>[3x]PF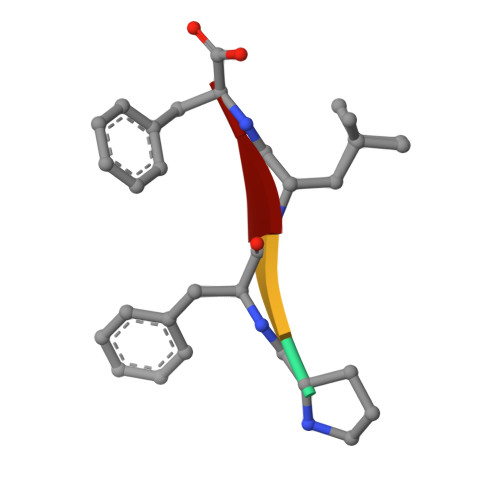LF Programmed formation of DNA double-strand breaks (DSBs) initiates the meiotic homologous recombination pathway. Meiotic DSBs are catalyzed by Spo11. Several other proteins are essential for meiotic DSB formation, including three evolutionarily conserved proteins first identified in Saccharomyces cerevisiae (Mer2, Mei4, and Rec114). Here, we show that mouse Rec114 is required for meiotic DSB formation.

Then, using limited trypsin proteolysis, we identified a stable fragment (residues 15–159) that was suitable for structural analysis. We determined the crystal structure of this REC114 N-terminal region at a resolution of 2.5 Å by SAD using the selenomethionine (SeMet)-substituted protein. The final model, refined to an Rfree of 30% and R-factor of 25% included residues 15–150. Unexpectedly, the structure revealed that REC114 (15-150) forms a PH domain, with two perpendicular antiparallel β-sheets followed by a C-terminal helix. Several residues are disordered in loops between the β strands. Mapping the conserved residues to the protein surface revealed that both β-sheets contained exposed conserved residues that could be involved in protein interactions with REC114 partners. In the crystal, the PH domain formed extensive crystallographic contacts with a symmetry-related molecule. Indeed, this interface, judged as significant using the PDBePisa server, buried a surface of 764 Å2 and included several salt bridges and hydrogen bonds formed by the well-conserved Arg98 of β6, and Glu130 and Gln137 of α1. When injected at lower concentrations, the protein eluted later and the molecular weight diminished (21 kD at 5 mg/ml). These results could be explained by a concentration-dependent dimerization of the PH domain with a fast exchange rate between monomers and dimers that co-purify together during SEC. Several conserved positively charged residues in the two β sheets, β1 and β2, important for the interaction are not present in REC114.

> AMGEVSQWSLKRYGRFMLLDNVGSPGPSSEAAAAGSPTWKVFESSEESGSLVLTIVVSGHFFISQGQTLLEGFSLIGSKNWLKIVRRMDCLLFGTTIKNKSRMFRVQFSGESKEEALERCCGCVQTLAQYVTVQEPDSTTQELQQSQ>DRHHHHHHKLNLTCPACKVLFTALNHGLKKEPNVARVGSVAIKICKMLNIAPLDVCQSAVHLFEDDVVEVWTRSVLSPSEACGLLLGSSCGHWDIFSTWNISLPSVPKPPPKPPSPPAPGAPVSRVLFLTDLHWDHEYLEGTDPYCADPLCCRRGSGWPPNSQKGAGFWGEYSKCDLPLRTLESLLKGLGPAGPFEMVYWTGDIPAHDVWQQSRQDQLRALTTITDL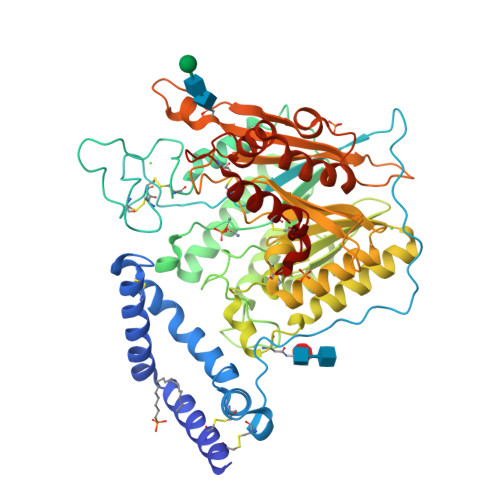VRKFLGPVPVYPAVGNHESTPVNGFPPPFIKGNQSSQWLYEAMAKAWEPWLPADALHTLRIGGFYALTPRPGLRLISLNMNFCSRENFWLLINSTDPAGQLQWLVEELQAAENRGDKVHIIGHIPPGHCLKSWSWNYYKIIARYENTLAGQFFGHTHVDEFEIFYDEETLSRPLAVAFLAPSATTFINLNPGYRVYQIDGNYPGSSHVVLDHETYILNLTQANAAGGTPSWKRLYRARETYGLPDAMPASWHNLVYRMRDDEQLFQTFWFLYHKGHPPSEPCGTPCRLATLCAQLSARADSPALCRHLMPN[4x]5-azanyl-3-[1-[[4-[(4-propan-2-ylpiperazin-1-yl)methyl]phenyl]methyl]indol-6-yl]-1~{H}-pyrazole-4-carbonitrile 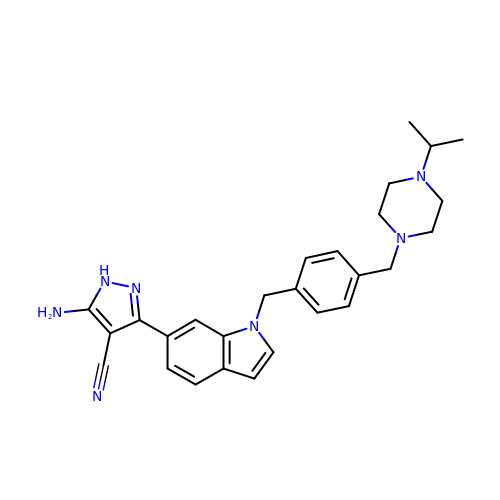| C27 H31 N7 | ZLJXHHAUABPXJM-UHFFFAOYSA-N methyl (2-{(R)-(3-chlorophenyl)[(3R)-1-({(2S)-1-(methylamino)-3-[(3R)-tetrahydro-2H-pyran-3-yl]propan-2-yl}carbamoyl)piperidin-3-yl]methoxy}ethyl)carbamate 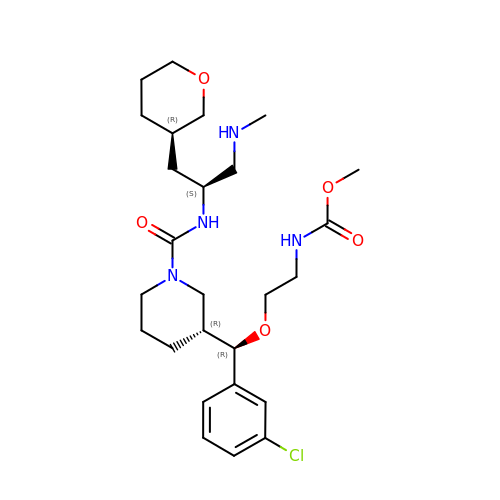| C26 H41 Cl N4 O5 | GCNDDOJRCKHYLZ-ZXMXYHOLSA-N>MPKKTIYFGAGWFTDRQNKAYKEAMEALKENPTIDLENSYVPLDNQYKGIRVDEHPEYLHDKVWATATYNNDLNGIKTNDIMLGVYIPDEEDVGLGMELGYALSQGKYVLLVIPDEDYGKPINLMSWGVSDNVIKMSQ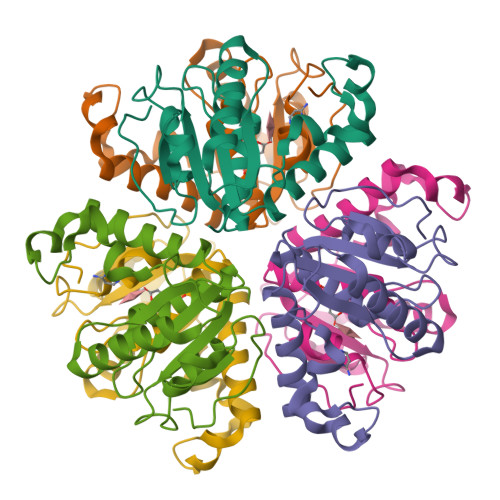LKDFNFNKPRFDFYEGAVY[2x]> MDFETNEDINGVRFTWNVFPSTRSDANSNVVPVGCLYTPLKEYDELNVAPYNPVVCSGPHCKSILNPYCVIDPRNSSWSCPICNSRNHLPPQYTNLSQENMPLELQSTTIEYITNKPVTVPPIFFFVVDLTSETENLDSLKESIITSLSLLPPNALIGLITYGNVVQLHDLSSETIDRCNVFRGDREYQLEALTEMLTGQKPTGPGGAASHLPNAMNKVTPFSLNRFFLPLEQVEFKLNQLLENLSPDQWSVPAGHRPLRATGSALNIASLLLQGCYKNIPARIILFASGPGTVAPGLIVNSELKDPLRSHHDIDSDHAQHYKKACKFYNQIAQRVAANGHTVDIFAGCYDQIGMSEMKQLTDSTGGVLLLTDAFSTAIFKQSYLRLFAKDEEGYLKMAFNGNMAVKTSKDLKVQGLIGHASAVKKTDANNISESEIGIGATSTWKMASLSPYHSYAIFFEIANTAANSNPMMSAPGSADRPHLAYTQFITTYQHSSGTNRIRVTTVANQLLPFGTPAIAASFDQEAAAVLMARIAVHKAETDDGADVIRWLDRTLIKLCQKYADYNKDDPQSFRLAPNFSLYPQFTYYLRRSQFLSVFNNSPDETAFYRHIFTREDTTNSLIMIQPTLTSFS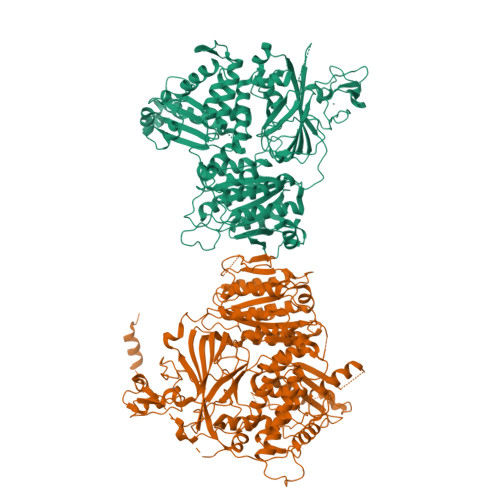MEDDPQPVLLDSISVKPNTILLLDTFFFILIYHGEQIAQWRKAGYQDDPQYADFKALLEEPKLEAAELLVDRFPLPRFIDTEAGGSQARFLLSKLNPSDNYQDMARGGSTIVLTDDVSLQNFMTHLQQVAVSGQA;> MSHHKKRVYPQAQLQYGQNATPLQQPAQFMPPQDPAAAGMSYGQMGMPPQGAVPSMGQQQFLTPAQEQLHQQIDQATTSMNDMHLHNVPLVDPNAYMQPQVPVQMGTPLQQQQQPMAAPAYGQPSAAMGQNMRPMNQLYPIDLLTELPPPITDLTLPPPPLVIPPERMLVPSELSNASPDYIRSTLNAVPKNSSLLKKSKLPFGLVIRPYQHLYDDIDPPPLNEDGLIVRCRRCRSYMNPFVTFIEQGRRWRCNFCRLANDVPMQMDQSDPNDPKSRYDRNEIKCAVMEYMAPKEYTLRQPPPATYCFLIDVSQSSIKSGLLATTINTLLQNLDSIPNHDERTRISILCVDNAIHYFKIPLDSENNEESADQINMMDIADLEEPFLPRPNSMVVSLKACRQNIETLLTKIPQIFQSNLITNFALGPALKSAYHLIGGVGGKIIVVSGTLPNLGIGKLQRRNESGVVNTSKETAQLLSCQDSFYKNFTIDCSKVQITVDLFLASEDYMDVASLSNLSRFTAGQTHFYPGFSGKNPNDIVKFSTEFAKHISMDFCMETVMRARGSTGLRMSRFYGHFFNRSSDLCAFSTMPRDQSYLFEVNVDESIMADYCYVQVAVLLSLNNSQRRIRIITLAMPTTESLAEVYASADQLAIASFYNSKAVEKALNSSLDDARVLINKSVQDILATYKKEIVVSNTAGGAPLRLCANLRMFPLLMHSLTKHMAFRSGIVPSDHRASALNNLESLPLKYLIKNIYPDVYSLHDMADEAGLPVQTEDGEATGTIVLPQPINATSSLFERYGLYLIDNGNELFLWMGGDAVPALVFDVFGTQDIFDIPIGKQEIPVVENSEFNQRVRNIINQLRNHDDVITYQSLYIVRGASLSEPVNHASAREVATLRLWASSTLVEDKILNNESYREFLQIMKARISK3-(1H-tetrazol-5-yl)-10lambda~6~-thioxanthene-9,10,10-trione | 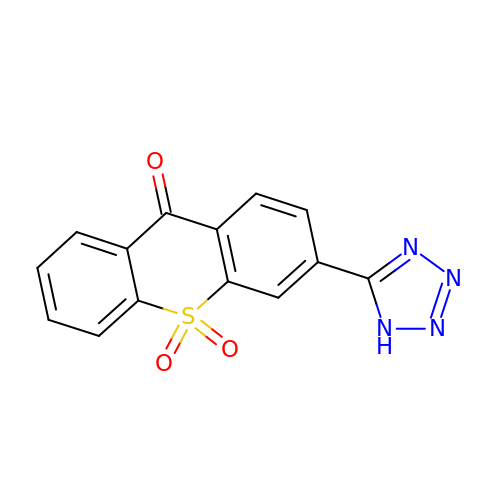C14 H8 N4 O3 S | VIDCTSLIEZMQRF-UHFFFAOYSA-N> 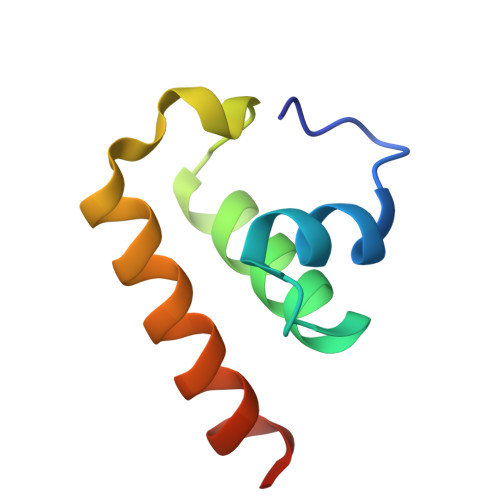MKITNDTTTYEVAELMGSEADELDGRIMMGLLSRECVVDTDDLSEDQWLALIDESQKVRREQFESDEA(2R)-2-(methoxymethyl)-4-(pyridin-2-yl)morpholine | C11 H16 N2 O2 | 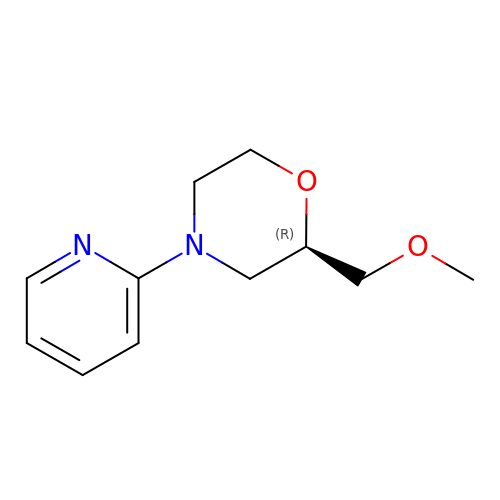QTYSPYFVCIFIBZ-SNVBAGLBSA-N> DEWSPMDPEEVAFEEAKCMEDHFGNDFGLAEKWMKWSLAESDGKTACYVKC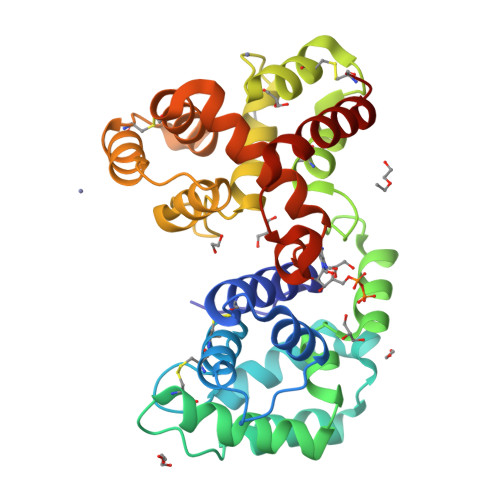LVEALGMYDKQAFQPNNIKQQYEAYKSDNGVDQTKGDAIANELGKIDAKDGKCESIAKGFIQVNNANKGVLEKIYLLDSSVRDAIYKKNPQIKPKGISIFRFCGKQFYQDGEAAYCNVRKHGFSDDPKFIKHSNCTTRGMRWMKKNGEMDESAILRGLHAVNENGKDDVVKKSLQNCKAKDESKARDYYKCIYDGLGEQLFMKVLDYIEVRSENYSYRLREATSKYDANAMRSKVKALDSEAKC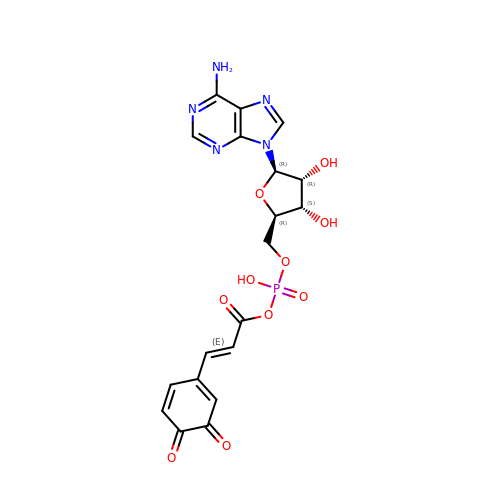5'-O-[(R)-{[(2E)-3-(3,4-dioxocyclohexa-1,5-dien-1-yl)prop-2-enoyl]oxy}(hydroxy)phosphoryl]adenosine | C19 H18 N5 O10 P | SRUDBSRTEMWJHC-LNTBVICDSA-N Rab GTPases play a crucial role in vesicular trafficking through shuttling between cytosol and membranes, a process that is controlled by several regulatory proteins. Another translocated effector protein LidA is also involved in the recruitment of early secretory vesicles to the LCV. LidA was found to interact with Rab1 as well, regardless of nucleotide binding states, and promote SidM/DrrA activity of transporting Rab1 to the LCV. Here, we present the crystal structures of LidA (residues 224-559) in complex with a GDP-bound Rab1 mutant (S25N; residues 1-176) and LidA (residues 188-449) in complex with GTP-bound Rab1 (residues 1-176).

To understand the underlying molecular mechanisms, we solved the crystal structure of LidA (residues 188-449) in complex with the Rab1(WT; residues 1-191) at 2.2 Å. The structure of the complex is highly similar to that of LidA(224-559)-Rab1(S25N) with an r.m.s.d of 0.678 Å for Rab1; 1.496 Å for LidA, respectively. As anticipated, GTP is well defined in the crystal structure and its interactions with Rab1 are conserved in other active Rabs. The hydrogen bonding interactions between the γ phosphate group of GTP with Thr43 and Gly69, from switch I and switch II of Rab1 respectively, are highly conserved among Rab proteins and important for stabilizing their active state. Our structural analyses suggest that LidA utilizes a similar mechanism to GTP for maintaining Rab1 in the active conformation. The GTP-Rab1-LidA structure shows truncation of the middle and the ring fingers does not disrupt Rab1-LidA complex, so that the thumb or the index fingers, though necessary, may not be sufficient to release Rab1. In the structure of GTP-Rab1-LidA we can see even the middle and the ring fingers are truncated, LidA can still holds Rab1. Deletion of the switch-stabilizing structural elements would be expected to disfavor LidA interaction with the GDP-bound Rab1 as compared to the GTP-bound Rab1. In support of the structure-based prediction, the assay showed that the LidA fragment exhibited a higher binding affinity (0.43 µM) to the GTP-bound Rab1 than to the GDP-bound Rab1 (2.4 µM).

> GPLGSMSSMNPEYDYLFKLLLIGDSGVGKSCLLLRFADDTYTESYISTIGVDFKIRTIELDGKTIKLQIWDTAGQERFRTITSSYYRGAHGIIVVYDVTDQESFNNVKQWLQEIDRYASENVNKLLVGNKCDLTTKKVVDYTTAKEFADSLGIPFLETSAKNATNVEQSFMTMAAEIKKRMGPGATAGGAEKSNVK;> GPLGSTSSTSQADKEIQKMLDEYEQAIKRAQENIKKGEELEKKLDKLERQGKDLEDKYKTYEENLEGFEKLLTDSEELSLSEINEKMKAFSKDSEKLTQLMEKHKGDEKTVQSLQREHHDIKAKLANLQVLHDAHTGKKSYVNEKGNPVSSLKDAHLAINKDQEVVEHKGQFYLLQKGQWDAIKNDPAALEKAQKDYSQSKHDLATIKMEALIHKLSLEMEKQLETINDLIMSTDPKENEEATKLLHKHNGLNLKLANLQDMLAVHR RNA exosomes are key players in degradation, processing, and quality control of a wide variety of RNA molecules and have a structurally conserved 9-subunit core common to eukarya and archaea. The common exosome core is composed of a hexameric ring of RNase PH subunits (Rrp41 and Rrp42 in archaea) capped on one side by three protein subunits containing RNA binding domains (Rrp4 and Csl4 in archaea). This architecture results in a barrel-like complex with a continuous central channel implicated in RNA binding in both archaea and eukarya. Whereas the archaeal exosome has an active phosphorolytic RNase PH core, eukaryotic exosomes rely on the additional hydrolytic RNAses Rrp44 and Rrp6 for activity.

To trap a complex of the archaeal exosome with Pi and RNA substrates bound at the active site, nonameric 3∗(Rrp41/Rrp42/Rrp4) complex from S. solfataricus with the D182A point mutation in the Rrp41 protein (Rrp41D182A) was used. This point mutation was previously shown to completely abolish RNase activity but is not directly involved in RNA or phosphate binding and presumably allows for both substrates to bind without being turned over. Rrp4/Rrp41D182A/Rrp42 mutant exosome crystallized in the cubic space group P213 with one copy of each subunit in the asymmetric unit and the full 9-subunit complex is generated by a crystallographic 3-fold axis. The density observed for the Pi in the 1.8 Å structure presented here is clearly tetrahedral (proving that Pi and not Cl− is bound) and facilitates accurate refinement of the four oxygen atom positions of the phosphate as well as determination of binding geometry. The small error of only 0.1 Å in coordinal positions for this structure (as estimated by the refinement program REFMAC) allows for accurate determination of the hydrogen bonding distances. This analysis reveals that the Pi ion is bound by four residues from the Rrp41 subunit. Specifically, the phosphate is coordinated by the side chains of R99, R139, and S138 as well as the main chain amino groups of G137, S138, and R139 (numbering according to the S. solfataricus sequence). A total of eight contacts with binding distances of 2.6–3.2 Å are observed creating a strong phosphate anion binding site. The two phosphate binding sites are almost identical and reveal very similar interactions between the protein and the phosphate. The position of the Pi-binding site is highly conserved between archaeal exosomes and RNase PH and PNPase enzymes indicating a conserved mechanism of phosphate-dependent RNA degradation among phosphorolytic exosome-like complexes.

> GHMSSTPSNQNIIPIIKKESIVSLFEKGIRQDGRKLTDYRPLSITLDYAKKADGSALVKLGTTMVLAGTKLEIDKPYEDTPNQGNLIVNVELLPLAYETFEPGPPDENAIELARVVDRSLRDSKALDLTKLVIEPGKSVWTVWLDVYVLDYGGNVLDACTLASVAALYNTKVYKVEQHSNGISVNKNEVVGKLPLNYPVVTISVAKVDKYLVVDPDLDEESIMDAKISFSYTPDLKIVGIQKSGKGSMSLQDIDQAENTARSTAVKLLEELKKHLGI;> GHMREMLQVERPKLILDDGKRTDGRKPDELRSIKIELGVLKNADGSAIFEMGNTKAIAAVYGPKEMHPRHLSLPDRAVLRVRYHMTPFSTDERKNPAPSRREIELSKVIREALESAVLVELFPRTAIDVFTEILQADAGSRLVSLMAASLALADAGIPMRDLIAGVAVGKADGVIILDLNETEAMWGEADMPIAMMPSLNQVTLFQLNGSMTPDEFRQAFDLAVKGINIIYNLEREALKSKYVEFKEEGV;> GHMNMSQSQEIVLQPRSIVVPGELLAEGEFQIPWSPYILKINSKYYSTVVGLFDVKDTQFEVIPLEGSFYYPKINDIVIGLVEDVEIYGWVVDIKAPYKAYLPASNLLGRSINVGEDLRRYLDVGDYVIARIENFDRSIDPVLSVKGKDLGRVSNGIVIDIMPVKVPRVIGKNKSMYETLTSKSGCSIFVANNGRIWATCPSRFSEEILIEAIRKIENESHIKGLTDRIKQFIEEKLGERNASSGETKTNS>MSELEKAMVALIDVFHQYSGREGDKHKLKKSELKELINNELSHFLEEIKEQEVVDKVMETLDNDGDGECDFQEFMAFVAMVT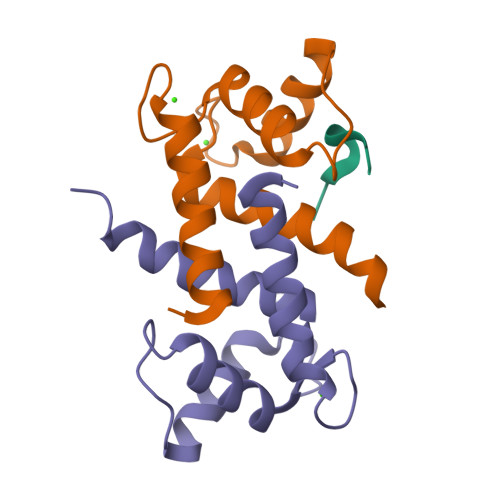TACHEFFEHE[4x];> NTGRTEAWKVLSPQG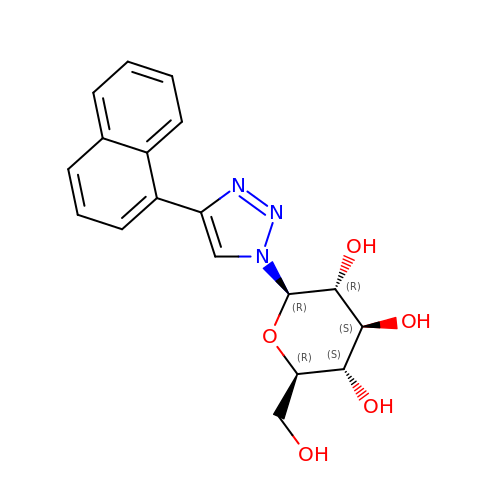1-beta-D-glucopyranosyl-4-naphthalen-1-yl-1H-1,2,3-triazole | C18 H19 N3 O5 | ZQSWMZLNZOWSSB-UYTYNIKBSA-N> PSVRPFKQRKSLAIRQEEVAGIRAKFPNKIPVVVERYPRETFLPPLDKTKFLVPQELTMTQFLSIIRSRMVLR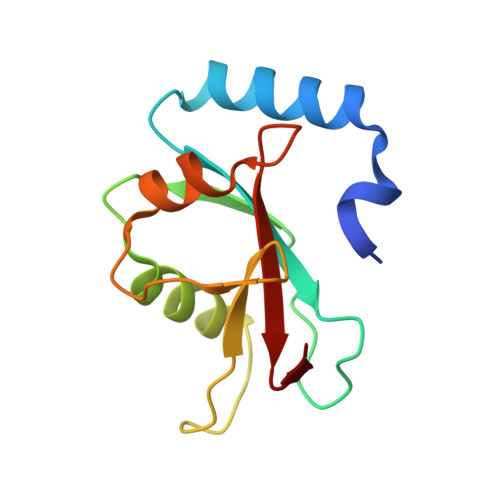ATEAFYLLVNNKSLVSMSATMAEIYRDYKDEDGFVYMTYASQETF>MAGARRLELGEALALGSGWRHVCHALLYAPDPGMLFGRIPLRYAILMQMRFDGRLGFPGGFVDTQDRSLEDGLNRELREELGEAAAAFRVERTDYRSSHVGSGPRVVAHFYAKRLTLEELLAVEAGATRAKDHGLEVLGLVRVPLYTLRDGVGGLPTFLENSFIGSAREQLLEALQDLGLLQSGSISGLKIPAHH[2x]

A similar cleavage reaction was observed in vitro with other enzymes from diverse organisms, including a snake venom phosphodiesterase (SVP), mammalian ectonucleotide pyrophosphatase/phosphodiesterase 1 (ENPP1), Escherichia coli RppH (EcRppH), and Homo sapiens NudT16 (HsNudT16). In addition, although NudT16 was initially characterized as a nucleolar U8 snoRNA decapping enzyme, it is involved in mRNA decapping and expresses across mouse tissues. Given the versatility in the recognition of substrates with diphosphate bonds, we and others have used some of these Nudix enzymes in vitro for processing ADP-ribosylation to a unique mass tag for site identification by tandem mass spectrometry (MS/MS). In this study, we sought to understand how HsNudT16 binds and hydrolyzes different forms of ADPr using X-ray crystallography.

Here we report the crystal structures of HsNudT16 in complex with ADPr and dimeric ADPr (di-ADPr). A 1″,2′-glycosidic linkage is observed between the first and second ADPr such that the latter subunit protrudes away from the substrate binding pocket. The second molecule (attached through C1) of ADPr does not make significant contacts to the Nudix fold beyond the mouth of HsNudT16. HsNudT16-di-ADPr structure suggests that the 2′-OH terminus of a PAR molecule is bound by the Nudix motif while the 1″-terminus, which is conjugated to proteins, is distal to the active site. Having said that, PARylated proteins would have even easier access to the HsNudT16 catalytic center with less steric hindrance than MARylated proteins where the latter would be closer to residues, such as Phe36′ and Phe61, at the mouth. In addition, the orientation of the PAR suggests a potential exonuclease activity from the 2′-OH terminus in concordance with the purported snoRNA decapping activity of HsNudT1660. However, since there is sufficient space to accommodate an additional ADPr linked to the 2′-OH terminus, we cannot exclude the possibility of endonuclease activity.>[4x]MAQENLQKIVDSLESSRAEREELYKWFHQHPEMSMQEHETSKRIAEELEKLGLEPQNIGVTGQVAVIKNGEGPSVAFRADFDALPITENTGLDYSADPELGMMHACGHDLHTTALLGAVRALVENKDLWSGTFIAVHQPGEEGGGGARHMVDDGLAEKIAAPDVCFAQHVFNEDPAFGYVFTPGRFLTAASNW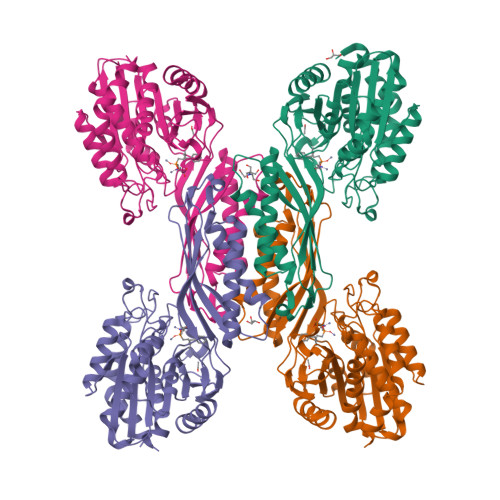RIHIHGEGGHGSRPHLTKDPIVVAASIITKLQTIVSREVDPNEVAVVTVGSIEGGKSTNSIPYTVTLGVNTRASNDELSEYVQNAIKRIVIAECQAAGIEQEPEFEYLDSVPAVINDEDLTEQLMAQFREFFGEDQAVEIPPLSGSEDYPFIPNAWGVPSVMWGWSGFAAGSDAPGNHTDKFAPELPDALERGTQAILVAAAPWLMK> MKKVRLKELESRLQQVDGFEKPKLLLEQYPTRPHIAACMLYTIHNTYDDIENK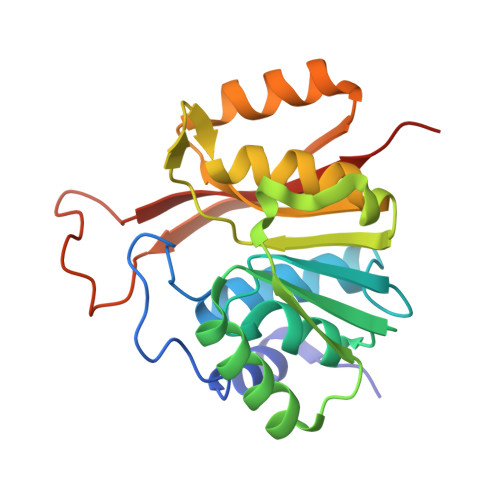VVADLGCGCGVLSIGTAMLGAGLCVGFDIDEDALEIFNRNAEEFELTNIDMVQCDVCLLSNRMSKSFDTVIMNPPFGTKNNKGTDMAFLKTALEMARTAVYSLHKSSTREHVQKKAAEWKIKIDIIAELRYDLPASYKFHKKKSVDIEVDLIRFSFHHHHHH>ISFKPGNQIDFNRLFTLPVTELFDPNTMFVYDQYVPLLVNLPSGFDQASIRLKVISYSVENQTLGVRLEFKDPQTQQFIPVLNASS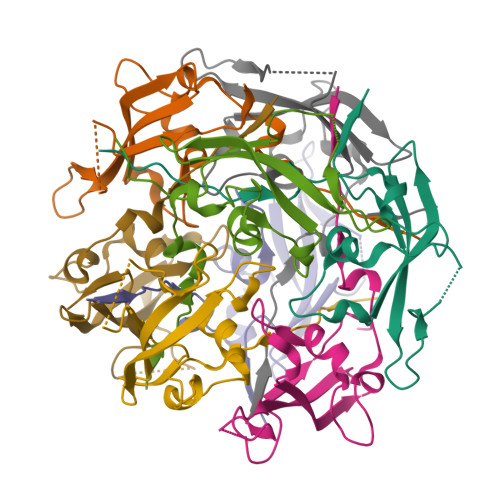TGPQTVFQPFNQWAD[8x]> LSKYGGECSKEHNTCTYRKDGKDHIVKCPSADNKKCKTDRHHCEYDDHHKTVDC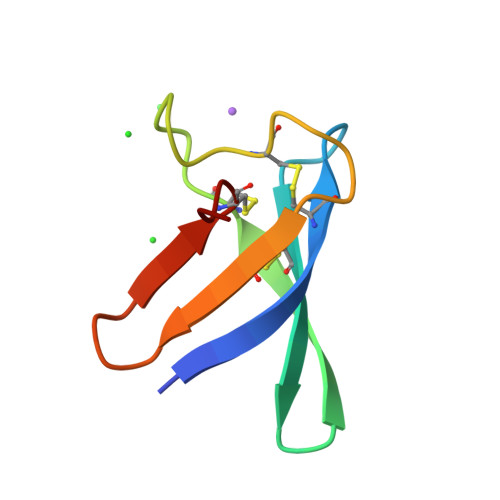QTPV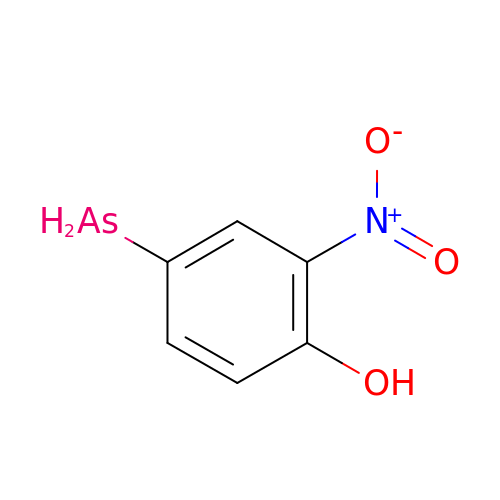4-arsanyl-2-nitrophenol | C6 H6 As N O3 | POYWCBSQXBGKKH-UHFFFAOYSA-N>HHHHHHFNLPPGNYKK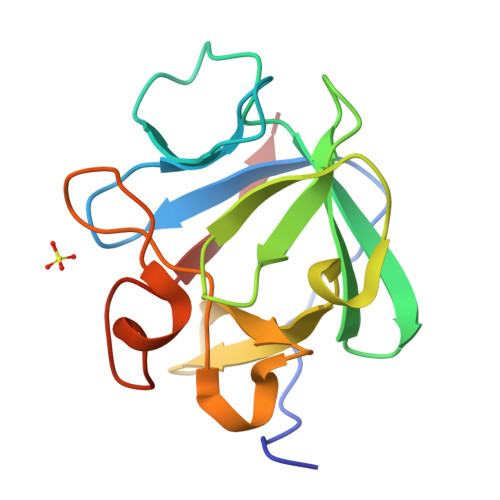PKLLYCSNGGHFLRINPDGTVDGTRDRSDQHIQLQLSAESVGEVYIKSTETGQYLAMDTDGLLYGSQTPNEECLFLERLEENHYNTYISKKHAEKNWFVGLKKNGSCKRGPRTHYGQKAILFLPLPVSSD[2x]>[8x]MSVSAFNRRWAAVILEALTRHGVRHICIAPGSRSTPLTLAAAENSAFIHHTHFDERGLGHLALGLAKVSKQPVAVIVTSGTAVANLYPALIEAGLTGEKLILLTADRPPELIDCGANQAIRQPGMFASHPTHSISLPRPTQDIPARWLVSTIDHALGTLHAGGVHINCPFAEPLYGEMDDTGLSWQQRLGDWWQDDKPWLREAPRLESEKQRDWFFWRQKRGVVVAGRMSAEEGKKVALWAQTL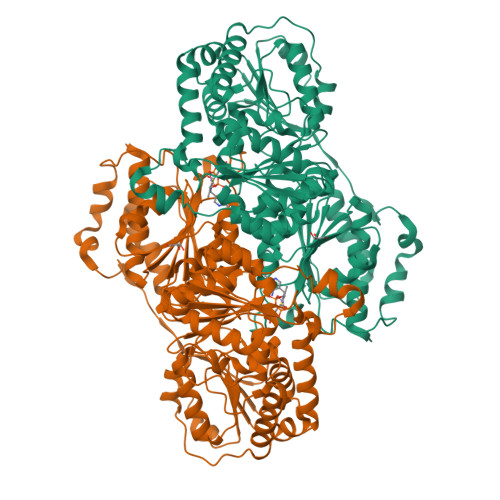GWPLIGDVLSQTGQPLPCADLWLGNAKATSELQQAQIVVQLGSSLTGKRLLQWQASCEPEEYWIVDDIEGRLDPAHHRGRRLIANIADWLELHPAEKRQPWCVEIPRLAEQAMQAVIARRDAFGEAQLAHRICDYLPEQGQLFVGNSLVVRLIDALSQLPAGYPVYSNRGASGIDGLLSTAAGVQRASGKPTLAIVGDLSALYDLNALALLRQVSAPLVLIVVNNNGGQIFSLLPTPQSERERFYLMPQNVHFEHAAAMFELKYHRPQNWQELETAFADAWRTPTTTVIEMVVNDTDGAQTLQQLLAQVSHL>VALVFAAEDVGSNKGAIIG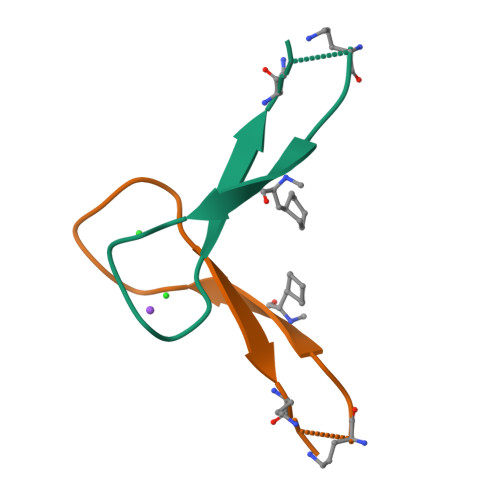LA[4x]> GAMDPDELPLDEH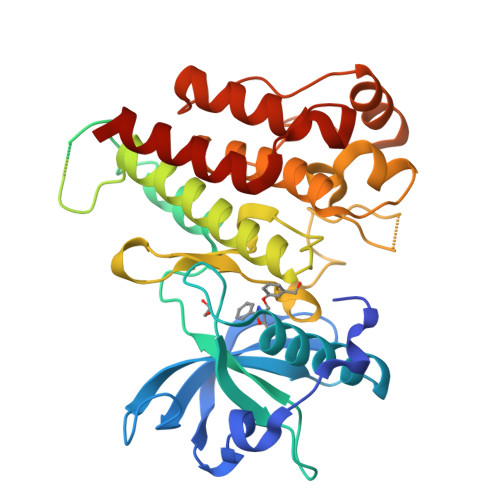CERLPYDASKWEFPRDRLKLGKPLGRGAFGQVIEADAFGIDKTATCRTVAVKMLKEGATHSEHRALMSELKILIHIGHHLNVVNLLGACTKPGGPLMVIVEFCKFGNLSTYLRSKRNEFVPYKTKGARFRQGKDYVGAIPVDLKRRLDSITSSQSSASSGFVEEKSLSDVEEEEAPEDLYKDFLTLEHLICYSFQVAKGMEFLASRKCIHRDLAARNILLSEKNVVKICDFGLARDIYKDPDYVRKGDARLPLKWMAPETIFDRVYTIQSDVWSFGVLLWEIFSLGASPYPGVKIDEEFCRRLKEGTRMRAPDYTTPEMYQTMLDCWHGEPSQRPTFSELVEHLGNLLQANAQQD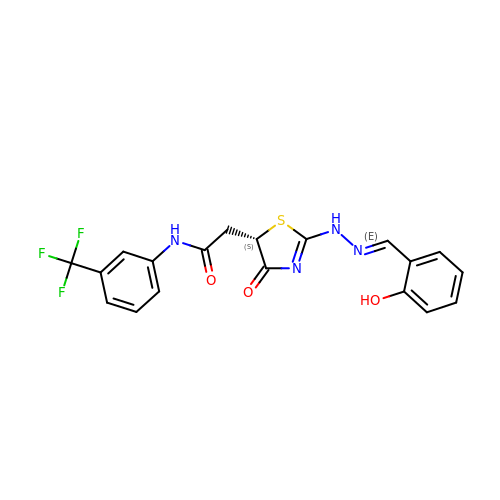2-{(5S)-2-[(2E)-2-(2-hydroxybenzylidene)hydrazinyl]-4-oxo-4,5-dihydro-1,3-thiazol-5-yl}-N-[3-(trifluoromethyl)phenyl]acetamide | C19 H15 F3 N4 O3 S | OBVIGUGYWMTZGZ-MQEPLNOPSA-N> HMASMKKKGSVVI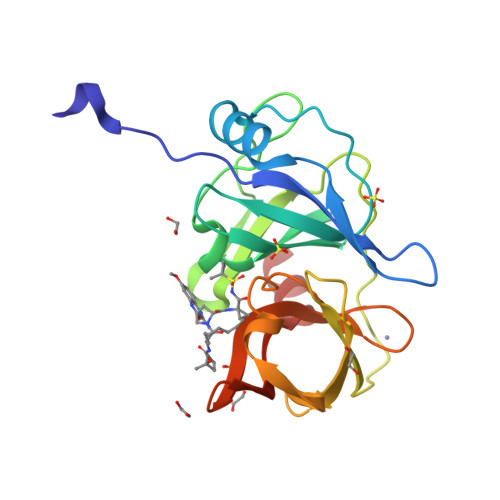VGRINLSGDTAYAQQTRGEEGCQETSQTGRDKNQVEGEVQIVSTATQTFLATSINGVLWTVYHGAGTRTIASPKGPVTQMYTNVDKDLVGWQAPQGSRSLTPCTCGSSDLYLVTRHADVIPVRRRGDSRGSLLSPRPISYLKGSSGGPLLCPAGHAVGIFRAAVSTRGVAKAVAFIPVESLETTMRSP>[2x]MVRLEDYGTWDEALKRLEASRK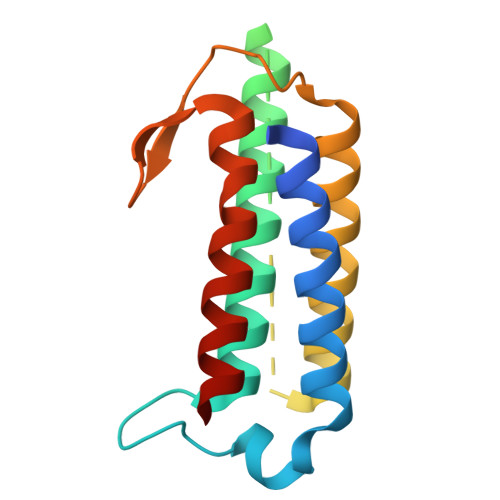ALLALLREADPAWLSAPLREGAWTPLMVAEHVALVEDSTARVLRRLRRLAAGENLPPVPVKPGEFKDGKPQAPEGVRPKGGLSLEEVLALLDRARAFLLEEVAKADPQNPATFPHPFFGELNPLGWLRAAAYHEAHHLKALQASLPR> SIKLQTNHGTITLKLFADKAPETAANFEQYVKDGHYDGTIFHRVIDGFMIQGGGFEPGMKQKSTRAPIKNEANNGLSNKKYTIAMARTPDPHSASAQFFINVKDNAFLDHTAP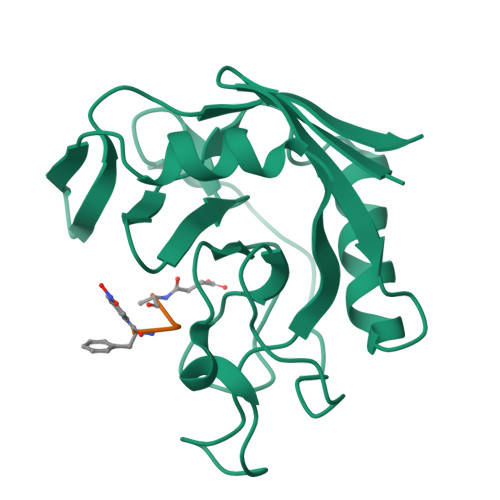TAHGWGYAVFGEVVEGTDVVDRIKSVATGSRAGHGDVPVDDVIIEKAEIV> SNAMESSTQTKPGSLIVVGTGIESIGQMTLQALSYIEAASKVFYCVIDPATEAFILTKNKNCVDLYQYYDNGKSRMDTYTQMAELMLKEVRNGLDVVGVFYGHPGVFVNPSHRALAIARSEGYQARMLPGVSAEDCLFADLCIDPSNPGCLTYEASDFLIRERPVNVHSHLILFQVGCVGIADFNFSGFDNSKFTILVDRLEQEYGPDHTVVHYIAAMMPHQ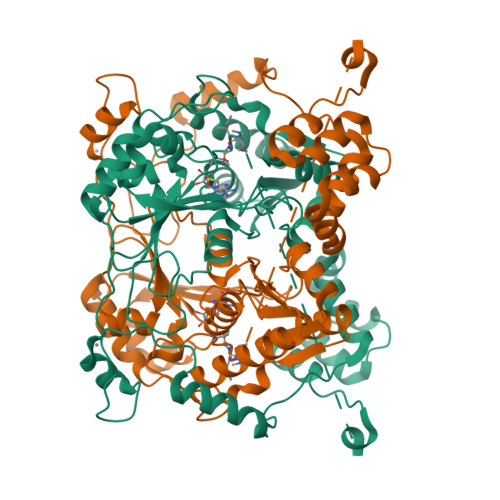DPVTDKFTIGQLREPEIAKRVGGVSTFYIPPKARKDINTDIIRLLEFLPAGKVPDKHTQIYPPNQWEPDVPTLPPYGQNEQAAITRLEAHAPPEEYQPLATSKAMTDVMTKLALDPKALAEYKADHRAFAQSVPDLTPQERAALELGDSWAIRCAMKNMPSSLLEAASQSVEEASMNGFPWVIVTGIVGVIGSVVSSA5-amino-1-[(4-bromo-2-fluorophenyl)methyl]-N-(2,5-dimethoxyphenyl)-1H-1,2,3-triazole-4-carboxamide 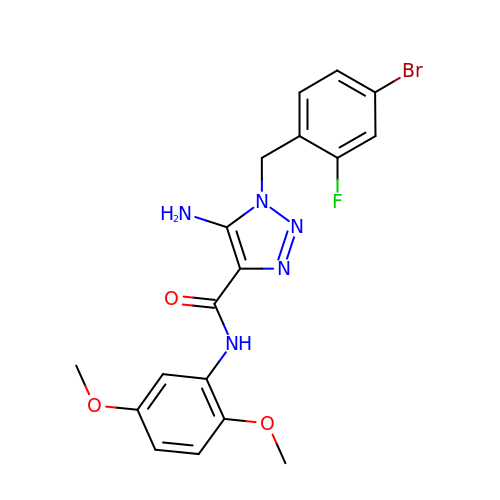| C18 H17 Br F N5 O3 | RAVNFJBKYUTEIC-UHFFFAOYSA-N> CPAYSXY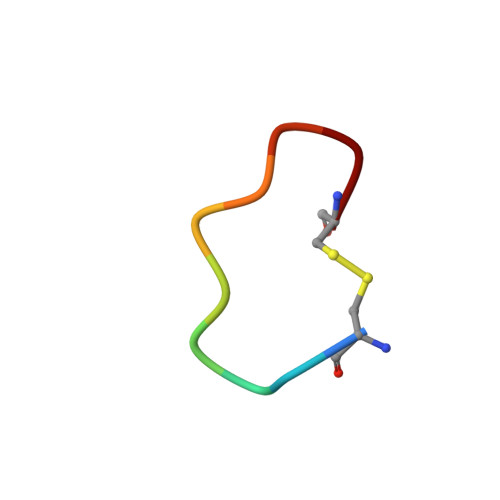LDC>[12x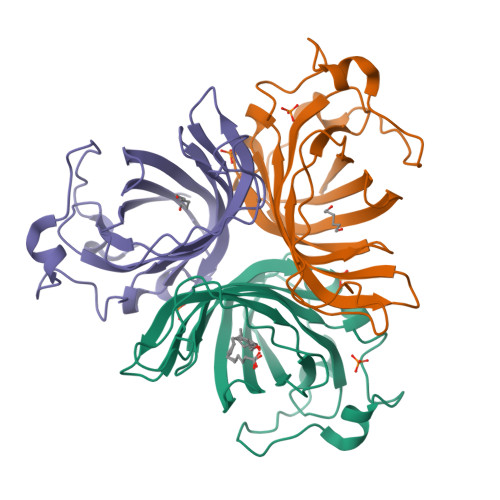]GGPLGSMAARGASPGHVQELFVYEINERDRGSPVFLPFGGKKQPGTDAHVNSLGDLVPFSNKIYDGSLKTRLGITAGLCTLISHSDQKNGDRYEALYSFYFGDYGHISVQGPYITYEDSYLAITGGSGIFAGCYGQAKLHQIIFPFKLFYTFYLQGIKKLPEALCAPCVPPSPSVAPADEAKQCLPNHVAPNFTK> MTTLLNPYFGEFGGMYVPQILMPALRQLEEAFVSAQKDPEFQAQFNDLLKNYAGRPTALTKCQNITAGTNTTLYLKREDLLHGGAHKTNQVLGQALLAKRMGKTEIIAETGAGQHGVASALASALLGLKCRIYMGAKDVERQSPNVFRMRLMGAEVIPVHSGSATLKDACNEALR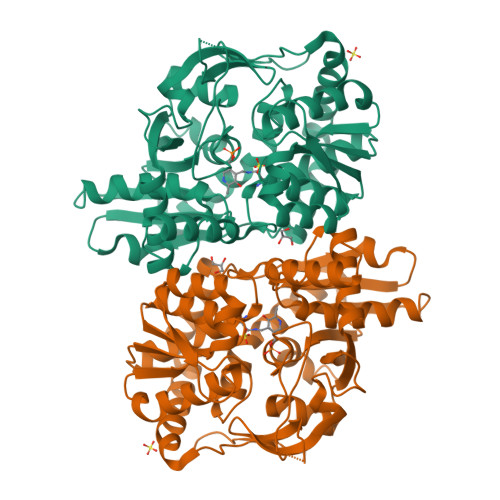DWSGSYETAHYMLGTAAGPHPYPTIVREFQRMIGEETKAQILEREGRLPDAVIACVGGGSNAIGMFADFINETNVGLIGVEPGGHGIETGEHGAPLKHGRVGIYFGMKAPMMQTEDGQIEESYSISAGLDFPSVGPQHAYLNSTGRADYVSITDDEALEAFKTLCLHEGIIPALESSHALAHALKMMRENPDKEQLLVVNLSGRGDKDIFTVHDILKARGEI> MKRIAFVFSTAPHGTAAGREGLDALLATSALTDDLAVFFIADGVFQLL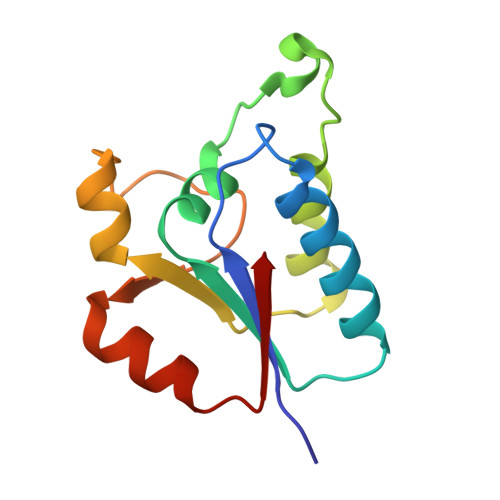PGQKPDAVLARDYIATFKLLGLYDIEQCWVCAASLRERGLDPQTPFVVEATPLEADALRRELANYDVILRF> MNARSTGQHPARYPGAAAGEPTLDSWQEPPHNRWAFAHLGEMVPSAAVSRRPVNAPGHALARLGAIAAQLPDLEQRLEQTYTDAFLVLRGTEVVAEYYRAGFAPDDRHLLMSVSKSLCGT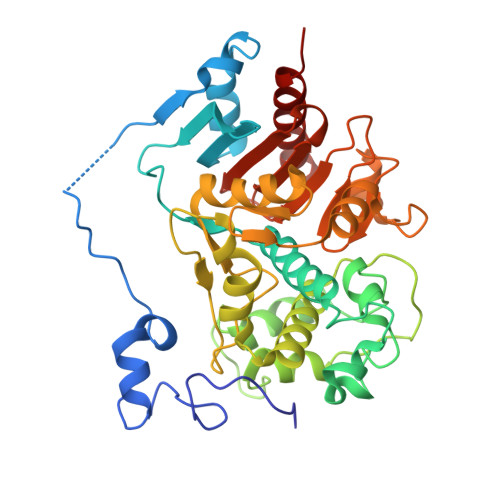VVGALVDEGRIDPAQPVTEYVPELAGSVYDGPSVLQVLDMQISIDYNEDYVDPASEVQTHGRSAGWRTRRHGDPADTYEFLTTLRGDGSTGEFQYCSANTDVLAWIVERVTGLRYVEALSTYLWAKLDADRDATITVDTTGFGFAHGGVSCTARDLARVGRMMLDGGVAPGGRVVSEDWVRRVLAGGSHEAMTDKGFTNTFPDGSYTRQWWCTGNERGNVSGIGIHGQNLWLDPLTDSVIVKLSSWPDPDTEHWHRLQNGILLDVSRALDAV>MAHHHHHHMASPASTNPAHDHFETFVQAQLCQDVLS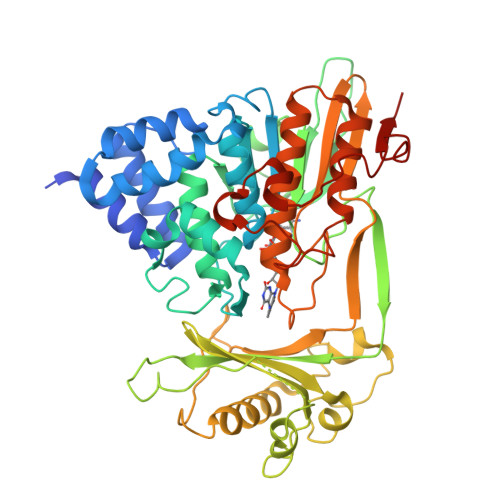SFQGLCRALGVESGGGLSQYHKIKAQLNYWSAKSLWAKLDKRASQPVYQQGQACTNTKCLVVGAGPCGLRAAVELALLGARVVLVEKRIKFSRHNVLHLWPFTIHDLRALGAKKFYGRFCTGTLDHISIRQLQLLLLKVALLLGVEIHWGVKFTGLQPPPRKGSGWRAQLQPNPPAQLASYEFDVLISAAGGKFVPEGFTIREMRGKLAIGITANFVNGRTVEETQVPEISGVARIYNQKFFQSLLKATGIDLENIVYYKDETHYFVMTAKKQCLLRLGVLRQDLSETDQLLGKANVVPEALQRFARAAADFATHGKLGKLEFAQDARGRPDVAAFDFTSMMRAESSARVQEKHGARLLLGLVGDCLVEPFWPLGTGVARGFLAAFDAAWMVKRWAEGAGPLEVLAERESLYQLLSQTSPENMHRNVAQYGLDPATRYPNLNLRAVTPNQVQDLYDMMDKE[2x]>GPGYQDPNNRYSFIGGRTGQWQVVKIRNVLGPGLQLVEKVNILNGAVAEIPLDSAWRLQGFASNIRYAIRTELEALQAVQPMLNRAEAILAVLIPIKKSAQWWEMAQDERRDIFERESHHTAVGLEYLPGV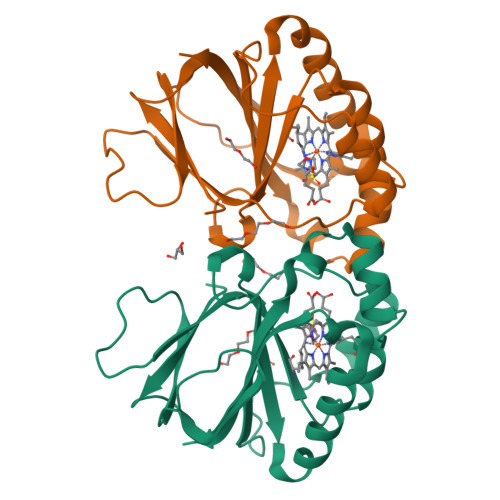AKRLLHCRDLGEEFDFLTWFEFAPEHSSAFNELLLRMRASKEWEYVEREVEVWLKRL[2x]>[2x]GPNLFVALYDFESRTENTLSITKGEKLRVLNNTENG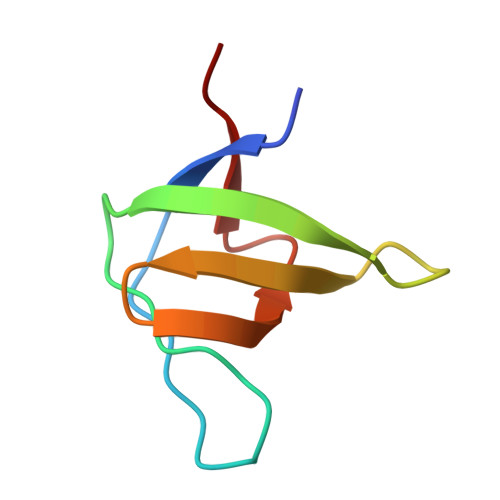EWCEAQTKNGQGWVPSNYITPVN> GGAAACCUGAUCAUGUAGAUCGAAUGGACUCUAAAUCCGUUCAGCCGGGUUAGA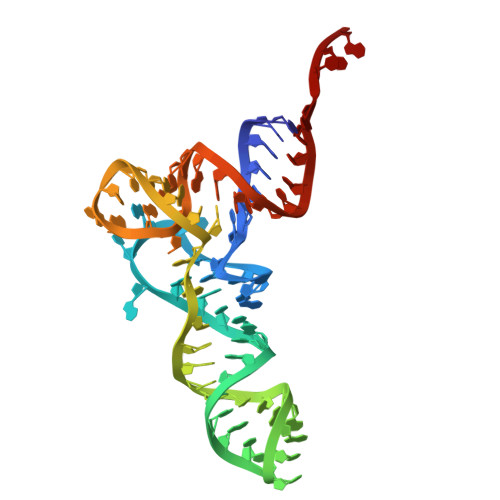UUCCCGGGGUUUCCGCCA>AMDPEFMREFQRAAVRLHILHHAADNEVHGAWLTQELSRHGYRVSPGTLYPTLHRLEADGLLVSEQRVVDGRARRVYRATPAGRAALTEDRRALEELAREV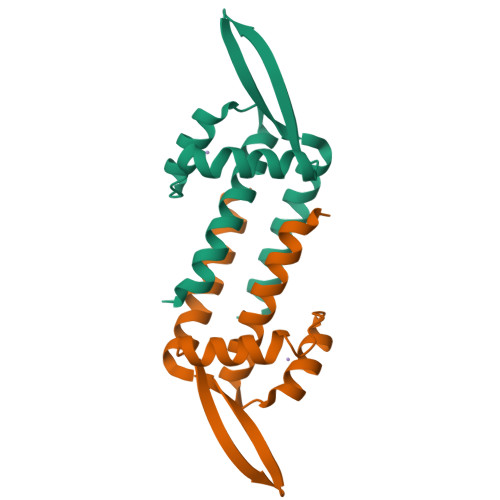LGGQSHTAGNGT[2x]> KKAIVDRSKAYVKLKSLGKEVRDAGYVPETKYVLHDI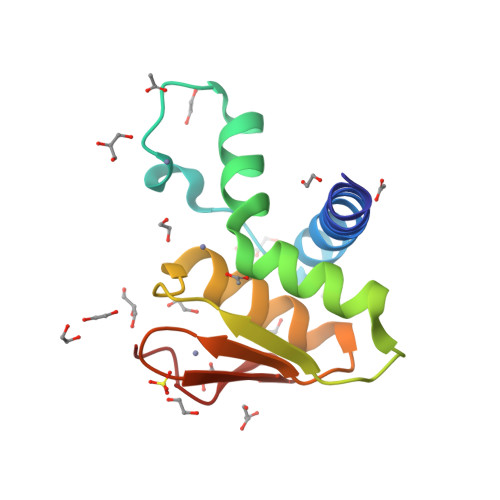DEEAKEKALMHHSERLAIAFGIINTPPGTTIRVMKNLRICGDCHNFIKILSSIEDREIIVRDNKRFHHFRDGNCSCGDYW>[2x]MTVAKKYLRLSVLTLVLSSFTLSAA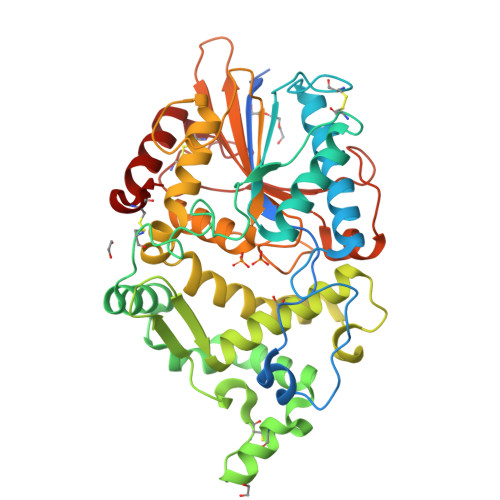PLAAQSTGYTLERVVILSRHGVRSPTKQTQLMNDVTPDKWPQWPVKAGYLTPRGAGLVTLMGGFYGDYFRSYGLLPAGCPADESIYVQADVDQRTRLTGQAFLDGIAPDCGLKVHYQADLKKIDPLFHTVEAGVCKLDPEKTHQAVEKRLGGPLNELSQRYAKPFALMGEVLNFSASPYCNSLQQKGKACDFATFAANEIEVNKEGTKVSLSGPLALSSTLGEIFLLQNSQAMPDVAWNRLSGEENWISLLSLHNAQFDLMAKTPYIARHKGTPLLQQIDTALVLQRDAQGQTLPLSPQTKLLFLGGHDTNIANIAGMLGANWQLPQQPDNTPPGGGLVFELWQNPDNHQRYVAVKMFYQTMEQLRNADKLDLKNNPARIVPIAIEGCENEGDNKLCQLETFQKKVAQVIEPSCHI BENZENE | C6 H6 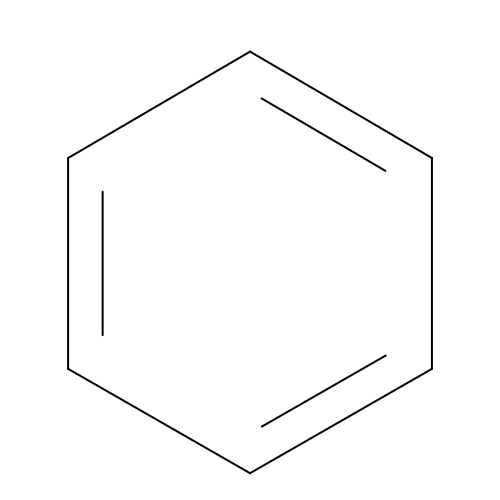| UHOVQNZJYSORNB-UHFFFAOYSA-N> PALPEDGGSGAFPPGHFKDPKRLYCKNGGFFLRIHPDGRVDGVREKSDPHIKLQLQAEERGVVSIKGVSANRYLAMKEDGRLLASKSVTD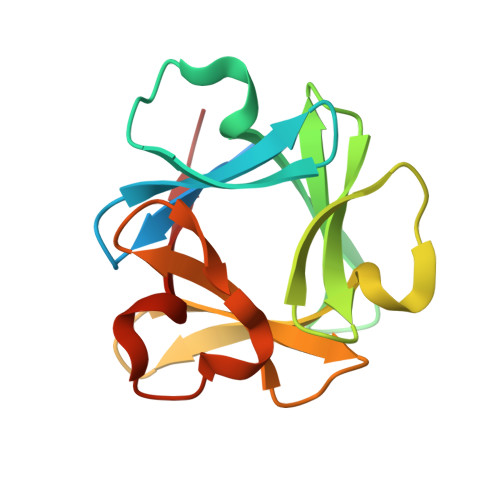ECFFFERLESNNYNTYRSRKYTSWYVALKRTGQYKLGSKTGPGQKAILFLPMSAKS> EQAKAQLSNGYNNPNVNASNMYGPPQNMSLPPPQTQTIQGTDQPYQYSQCTGRRKALIIGINYIGSKNQLRGCINDAHNIFNFLTNGYGYSSDDIVILTDDQNDLVRVPTRANMIRAMQWLVKDAQPNDSLFLHYSGHGGQTEDLDGDEEDGMDDVIYPVDFETQGPIIDDEMHDIMVKPLQQGVRLTALFDSAHSGTVLDLPYTYSTKGIIKEPNIWKDVGQDGLQAAISYATGNRAALIGSLGSIFKTVKGGMGNN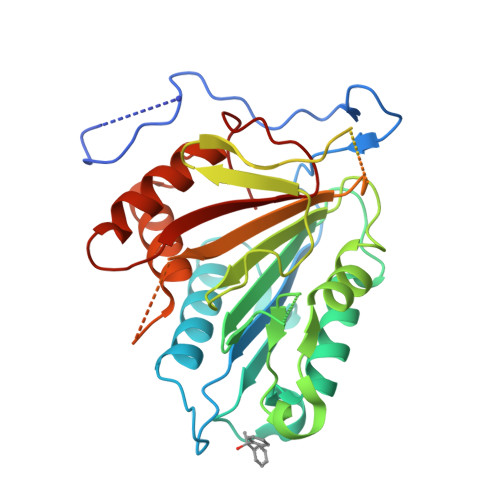VDRERVRQIKFSAADVVMLSGSKDNQTSADAVEDGQNTGAMSHAFIKVMTLQPQQSYLSLLQNMRKELAGKYSQKPQLSSSHPIDVNLQFIM> MLNPIVRKFQYGQHTVTLETGMMARQATAAVMVSMDDTAVFVTVVGQKKAKPGQDFFPLTVNYQERTYAAGRIPGSFFRREGRPSEGETLIARLIDRPVRPLFPEGFVNEVQVIATVVSVNPQVNPDIVAMIGASAALSLSGIPFNGPIGAARVGYINDQYVLNPTQDELKESKLDLVVAGTEAAVLMVESEAELLSEDTMLGAV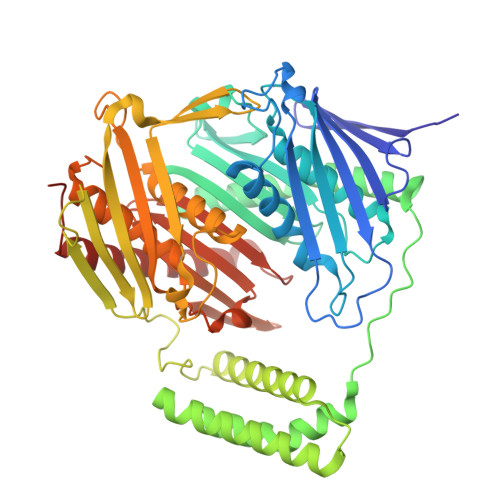VFGHEQQQVVIQAINDLVKEAGKPRWDWQPEAVNDALNARVAALAESRLSDAYRITDKQERYAQVDVIKSETIEQLIAEDETLDANELGEILHAIEKNVVRSRVLAGEPRIDGREKDMIRGLDVRTGVLPRTHGSALFTRGETQALVTATLGTARDAQVLDELMGERTDSFLFHYNFPPYSVGETGMVGSPKRREIGHGRLAKRGVLAVMPDMDKFPYTVRVVSEITESNGSSSMASVCGASLALMDAGVPIKAAVAGIAMGLVKEGDNYVVLSDILGDEDHLGDMDFKVAGSRDGISALQMDIKIEGITKEIMQVALNQAKGARLHILGVMEQAINAPRG~{N},~{N}-dimethyl-1~{H}-pyrazole-4-sulfonamide | C5 H9 N3 O2 S | 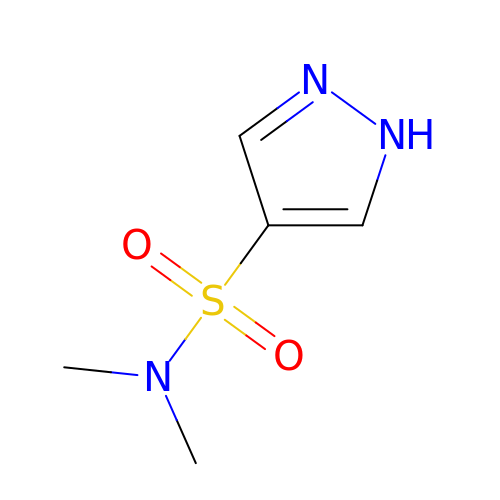HEIPZBCMZXCIPT-UHFFFAOYSA-N>[2x]MPPRFNIANVLLSPDGETFFRGFRSKIHAKGSLVCTGEGDENGVFVVVDGRLRVYLVGEEREISLFYLTSGDMFCMH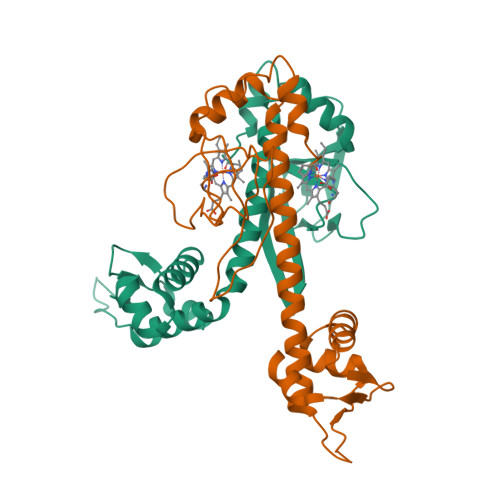SGCLVEATERTEVRFADIRTFEQKLQTCPSMAWGLIAILGRALTSCMRTIEDLMFHDIKQRIAGFFIDHANTTGRQTQGGVIVSVDFTVEEIANLIGSSRQTTSTALNSLIKEGYISRQGRGHYTIPNLVRLKAAADGDRDDDDD>[4x]MELLKEKLVLVTGAGRGLGAAISSGAAEQGARVILVDIDGTAAKAQADALTAKGFVAEGHALDVTDRDAVAALADDILSRFGGLDVLVNNAGVAGR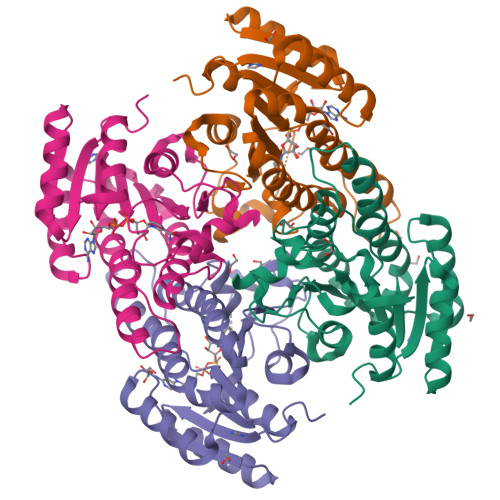AAFDQPEAVEVWDRVIGVNLEGAFNVSHALVPALKAAKGNVVHLCSVAGFVSGGSTAGYVVSKGAIRSLTQVMARDLAPHGIRVNAVAPGIMMSEMAVAQLNRPGGTDWFMNRVMMKRIGETSEVVDPVVFLASPMASYITGTILPVDGGFLAA>KKLNLKDKYQYLTRDMAWEPTYQDKKDIFPEEDFEGIKITDWSQWEDPFRLTMDAYWKYQAEKEKKLYAIFDAFAQNNGHQNISDARYVNALKLFISGISPLEHAAFQGYSKVGRQFSGAGARVACQMQAIDELRHSQTQQHAMSHYNKHFNGLHDGPHMHDRVWYLSVPKSFFDDARSAGPFEFLTAISFSFEYVLTNLLFVPFMSGAAYNGDMATVTFGFSAQSDEARHMTLGLEVIKFILEQHEDNVPIVQRWIDKWFWRGFRLLSLVSMMMDYMLPNKVMSWSEAWEVYYEQNGGALFKDLERYGIRPPKYQDVANDAKHHLSHQLWTTFYQYCQATNFHTWIPEKEEMDWMSEKYPDTFDKYYRPRYEYLAKEAAAGRRFYNNTLPQLCQVCQIPTIFTEKDAPTMLSHRQIEHEGERYHFCSDGCCDIFKHEPEKYIQAWLPVHQIYQGNCEGGDLETVVQKYYHINIGEDNFDYVGSPDQKHWLSIK[2x];>EIKTNSVEPIRHTYGHIARRFGDKPATRYQEASYDIEAKTNFHYRPQWDSEHTLNDPTRTAIRMEDWCAVSDPRQFYYGAYVGNRAKMQESAETS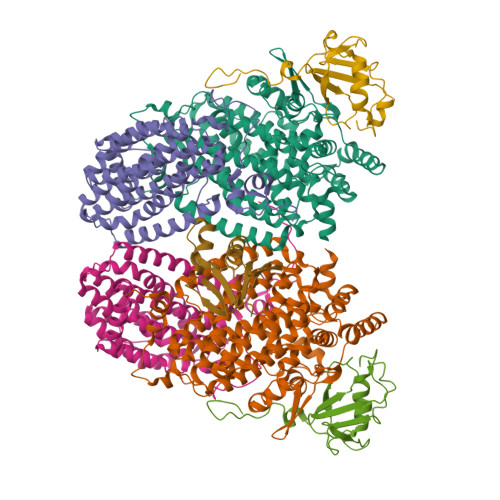FGFCEKRNLLTRLSEETQKQLLRLLVPLRHVELGANMNNAKIAGDATATTVSQMHIYTGMDRLGIGQYLSRIALMIDGSTGAALDESKAYWMDDEMWQPMRKLVEDTLVVDDWFELTLVQNILIDGMMYPLVYDKMDQWFESQGAEDVSMLTEFMRDWYKESLRWTNAMMKAVAGESETNRELLQKWIDHWEPQAYEALKPLAEASVGIDGLNEARAELSARLKKFELQSRGV[2x];>[2x]SVNALYDYKFEPKDKVENFHGMQLLYVYWPDHLLFCAPFALLVQPGMTFSALVDEILKPATAAHPDSAKADFLNAEWLLNDEPFTPKADASLKEQGIDHKSMLTVTTPGLKGMANAGY;> MSQLVFIVFQDNDDSRYLAEAVMEDNPDAEMQHQPAMIRIQAEKRLVINRETMEEKLGRDWDVQEMLINVISIAGNVDEDDDHFILEWN>[3x]GSGGSIRLADLAQQLDAELHGDGDIVITGVASMQSAQTGHITFMVNPKYREHLG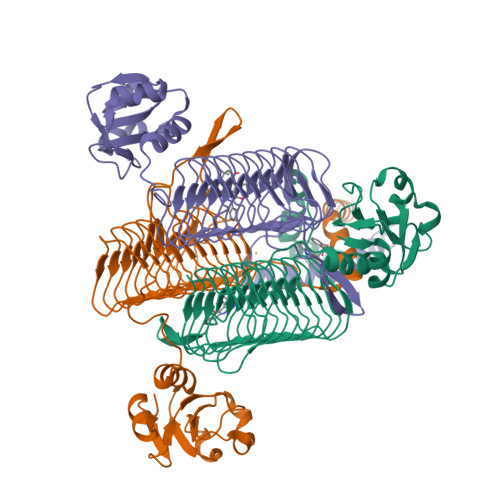LCQASAVVMTQDDLPFAKSAALVVKNPYLTYARMAQILDTTPQPAQNIAPSAVIDATAKLGNNVSIGANAVIESGVELGDNVIIGAGCFVGKNSKIGAGSRLWANVTIYHEIQIGQNCLIQSGTVVGADGFGYANDRGNWVKIPQIGRVIIGDRVEIGACTTIDRGALDDTIIGNGVIIDNQCQIAHNVVIGDNTAVAGGVIMAGSLKIGRYCMIGGASVINGHMEICDKVTVTGMGMVMRPITEPGVYSSGIPLQPNKVWRKTAALVMNIDDMSKRLKSLERKVNQQD2-[(naphthalen-2-yl)oxy]-5-(1H-pyrazol-4-yl)benzoic 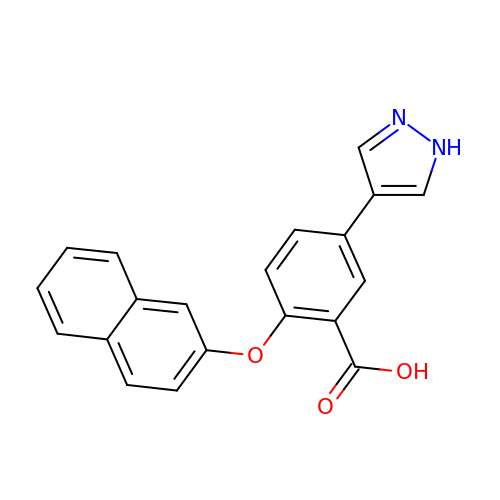acid | C20 H14 N2 O3 | CKJXZYIEHQOLFR-UHFFFAOYSA-N> SGIVQQQNNLLRAIEAQQHLLQLTVWAI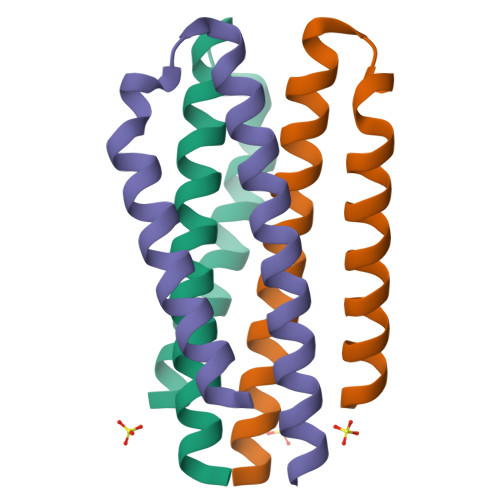KQLQARSGGRGGWMEWDREINNYTSLIHSLIEESQNQQEK>[2x]SMSGISPKKSKYMTPMQQKLNEVY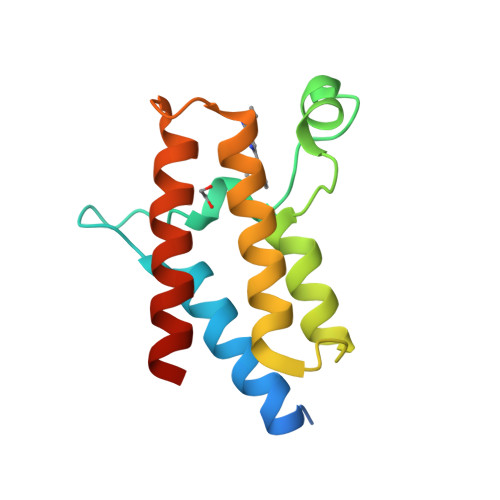EAVKNYTDKRGRRLSAIFLRLPSRSELPDYYLTIKKPMDMEKIRSHMMANKYQDIDSMVEDFVMMFNNACTYNEPESLIYKDALVLHKVLLETRRDLEGD>GPSRKTYTLTDYLKNTYRLKLYSLRWISDHEYLYKQENNILVFNAEYGNSSVFLENSTFDEFGHSINDYSISPDGQFILLEYNYVKQWRHSYTASYDIYDLNKRQLITEERIPNNTQWVTWSPVGHKLAYVWNNDIYVKIEPNLPSYRITWTGKEDIIYNGITDWVYEEEVFSAYSALWWSPNGTFLAYAQFNDTEVPLIEYSFYSDESLQYPKTVRVPYPKAGAVNP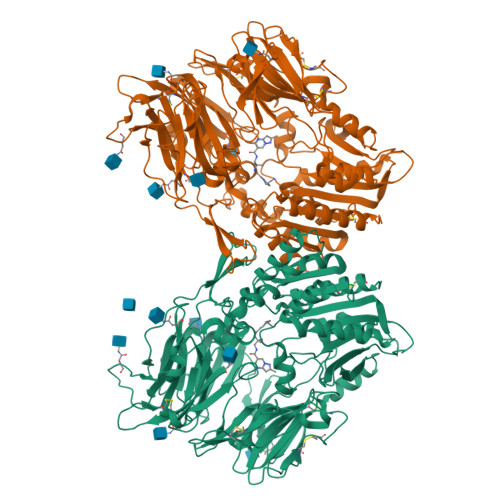TVKFFVVNTDSLSSVTNATSIQITAPASMLIGDHYLCDVTWATQERISLQWLRRIQNYSVMDICDYDESSGRWNCLVARQHIEMSTTGWVGRFRPSEPHFTLDGNSFYKIISNEEGYRHICYFQIDKKDCTFITKGTWEVIGIEALTSDYLYYISNEYKGMPGGRNLYKIQLSDYTKVTCLSCELNPERCQYYSVSFSKEAKYYQLRCSGPGLPLYTLHSSVNDKGLRVLEDNSALDKMLQNVQMPSKKLDFIILNETKFWYQMILPPHFDKSKKYPLLLDVYAGPCSQKADTVFRLNWATYLASTENIIVASFDGRGSGYQGDKIMHAINRRLGTFEVEDQIEAARQFSKMGFVDNKRIAIWGWSYGGYVTSMVLGSGSGVFKCGIAVAPVSRWEYYDSVYTERYMGLPTPEDNLDHYRNSTVMSRAENFKQVEYLLIHGTADDNVHFQQSAQISKALVDVGVDFQAMWYTDEDHGIASSTAHQHIYTHMSHFIKQCFSLP[2x]>MADPGDRLGVLTTTRRVVEQAQAVWIDHDAVAQIAEAFAARQVTPPTWNRELHWSDGREALANYILVLDAVNFCFWGEPR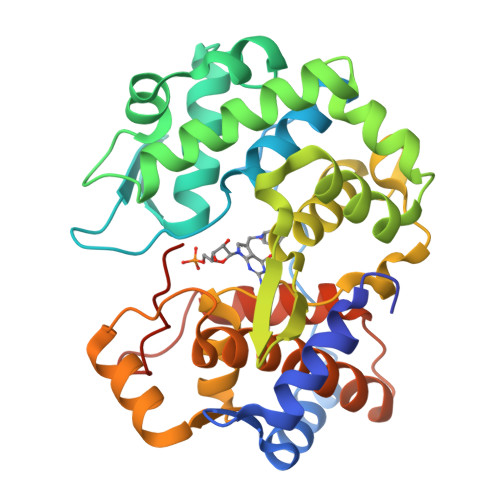WRIEYAGAVYDGYWALAASLKRALEQGVPLTDASYLAEITRDDVATIFAGEGEIPLLDERARILRETGSVLAERFAGRFSDAIAAAGRSAVALVDIVTNAFPSFRDVATYRGEQVRFYKRAQILVSDLYGAFDGSDLGAFDDLGELTAFANYKVPQVLHHLGILRYAPALHDRLARREEIPAGSPEEVEIRAATIWGVEELRRALASRGHALDAYQVDWLLWDEGQRLPAGTLPYHRTRTIFYLEHHHHHH[2x]>VSEDLRSRIEVLKRKVIEKVQHIQLLQKNVRAQLVDMKRLEVDIDIKIRSCRGSCSRALAREVDLKDYEDQQKQLEQVIAKDLLPSR[2x];>DNENVVNEYSSELEKHQLYIDETVNSNIPTNLRVLRSILENLRSKIQKLESDVSAQMEYCRTPCTVSCNIPVVSGKECEEIIRKGGETSEMYLIQPDSSVKPYRVYCDMNTENGGWTVIQNRQDGSVDFGRKWDPYKQGFGNVATNTDGKNYCGLPGEYWLGNDKISQLTRMGPTELLIEMEDWKGDKVKAHYGGFTVQNEANKYQISVNKYRGTAGNALMDGASQLMGENRTMTIHNGMFFSTYDRDNDGWLTSDPRKQCSKEDGGGWWYNRCHAANPNGRYYWGGQYTWDMAKHGTDDGVVWMNWKGSWYSMRKMSMKIRPFFPQQ[2x];>MLEEIMKYEASILTHDSSIRYLQEIYNSNNQKIVNLKEKVAQLEAQCQEPCKDTVQIHDITGKDCQDIANKGAKQSGLYFIKPLKANQQFLVYCEIDGSGNGWTVFQKRLDGSVDFKKNWIQYKEGFGHLSPTGTTEFWLGNEKIHLISTQSAIPYALRVELEDWNGRTSTADYAMFKVGPEADKYRLTYAYFAGGDAGDA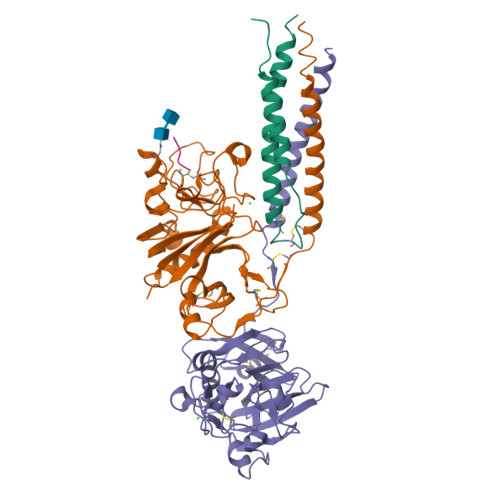FDGFDFGDDPSDKFFTSHNGMQFSTWDNDNDKFEGNCAEQDGSGWWMNKCHAGHLNGVYYQGGTYSKASTPNGYDNGIIWATWKTRWYSMKKTTMKIIPFNRLTIGEGQQHHLGGAKQAGDV[2x];>AHRPX[2x]>[12x]MSKTESYCLEDALNDLFIPETTIETILKRLTIKKNIILQGPPGVGKTFVARRLAYLLTGEKAPQRVNMVQFHQSYSYEDFIQGYRPNGVGFRRKDGIFYNFCQQAKEQPEKKYIFIIDEINRANLSKVFGEVMMLMEHDKRGENWSVPLTYSENDEERFYVPENVYIIGLMNTADRSLAVVDYALRRRFSFIDIEPGFD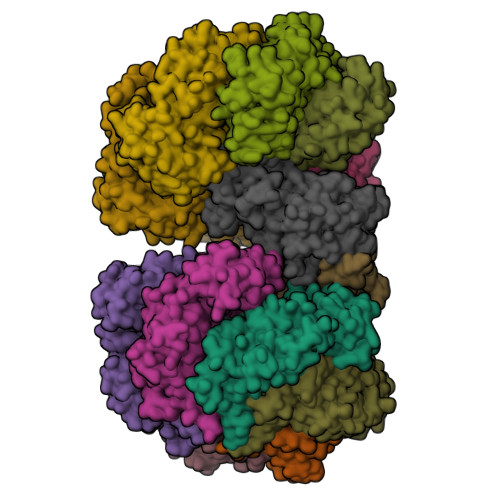TPQFRNFLLNKKAEPSFVESLCQKMNELNQEISKEATILGKGFRIGHSYFCCGLEDGTSPDTQWLNEIVMTDIAPLLEEYFFDDPYKQQKWTNKLLGDSSGSHHHHHH;>MEQPVIPVRNIYYMLTYAWGYLQEIKQANLEAIPGNNLLDILGYVLNKGVLQLSRRGLELDYNPNTEIIPGIKGRIEFAKTIRGFHLNHGKTVSTFDMLNEDTLANRIIKSTLAILIKHEKLNSTIRDEARSLYRKLPGISTLHLTPQHFSYLNGGKNTRYYKFVISVCKFIVNNSIPGQNKGHYRFYDFERNEKEMSLLYQKFLYEFCRRELTSANTTRSYLKWDASSISDQSLNLLPRMETDITIRSSEKILIVDAKYYKSIFSRRMGTEKFHSQNLYQLMNYLWSLKPENGENIGGLLIYPHVDTAVKHRYKINGFDIGLCTVNLGQEWPCIHQELLDIFDEYLK[2x]> GPMIDLYTAATPNGHKVSIALEEMGLPYTVHALSFDKKEQKAPEFLRINPNG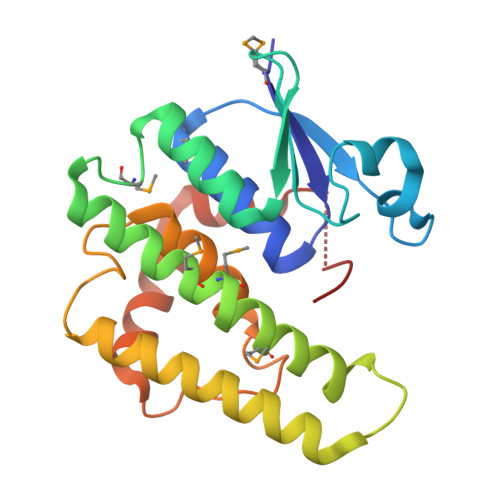RIPAIVDRSNDDFAVFESGAILVYLAEKTGQLMPTDVKGRSRVIQWLMFQMGGVGPMQGQANVFFRYFPEKLQGAIDRYQHETRRLYEVLDGRLGEAEYLAGDYSIADIATYPWVRIHDWSGVAVDGLDNLQRWIAALEARPAVQRGLLVPRREKEGDDAIR>APLAQADTPSSPSIDQVEPYSSTAQVQFDEPEATGGVPILKYKAEWRAVGEEVWHSKWYDAKEASMEGIVTIVGLKPETTYAVRLAALNGKGLGEISAASEFKTQPVREPSAPKLEGQRGEDGNSIKVNLIKQDDGGSPIRHYLVRYRALSSEWKPEIRLPSGSDHVMLKSLDWNAEYEVYVVAENQQGKSKAAHFVFRTAAAHH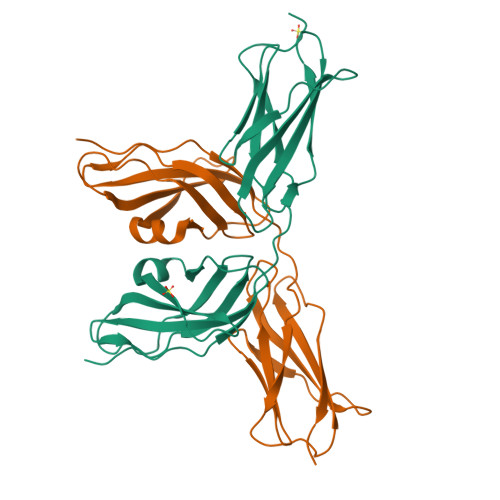HHHH[6x]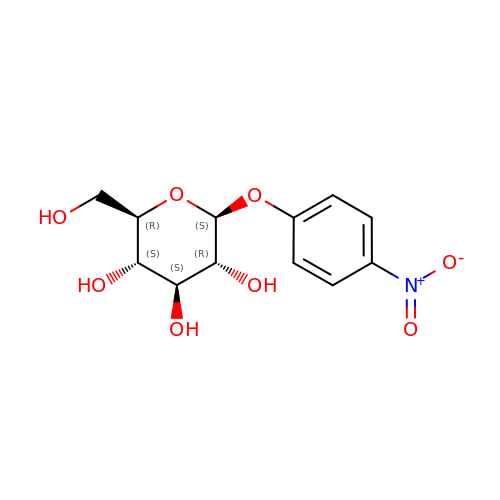4-nitrophenyl beta-D-glucopyranoside | C12 H15 N O8 | IFBHRQDFSNCLOZ-RMPHRYRLSA-N> MTREELLRENIELAKEHIEIMR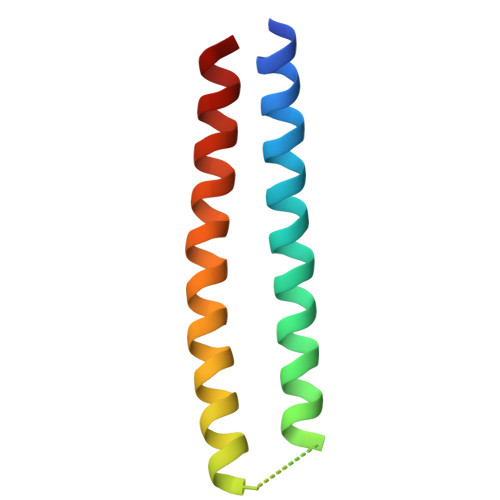EILELLQKMEELLEKARGADEDVAKTIKELLRRLKEIIERNQRIAKEHEYIARERS> PEEERIKYVITVVEQIAKDAHRNGQEELAKLAERTAEEAKKATERGEEETLRIVYVIVVVLQIALEAHRNGQEELAKLALRTAEEAIKATERGEEETLRIVYVIVVVLQIALEAHRNGQEELAKLALRTAEEAIKATERGEEETLRIVYVIVVVLQIALEAHRNGQEELAKLALRTAEEAIK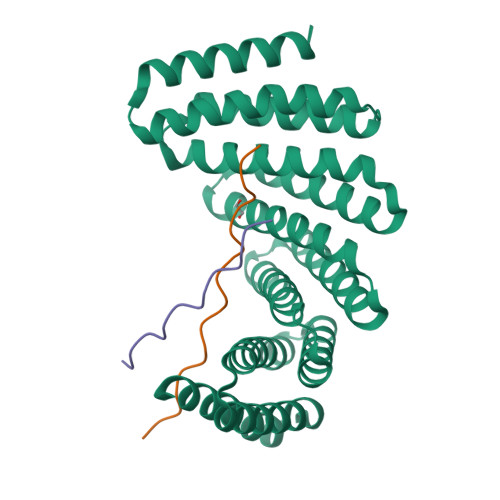ATERGEEETLRIVYVIVVVLQIALEAHRNGQEELAKLALRTAEEAIKATERGEEETERIVYDIVVVLQEALEAHRNGEEERAKKALDEARRRIEATERGE;>PLPPLPPLPPLPPLPPLPPLP[2x]> PRGLGPLQIWQTDFTLEPRMA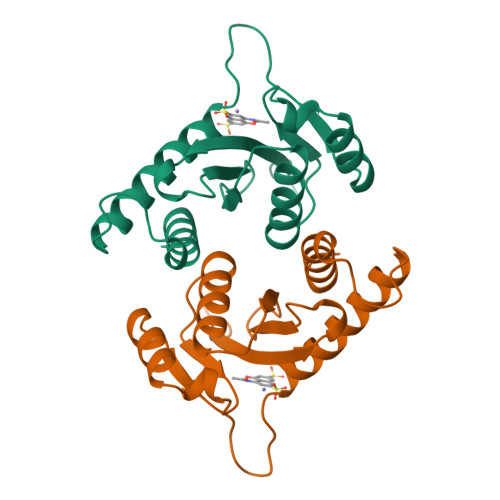PRSWLAVTVDTASSAIVVTQHGRVTSVAAQHHWATAIAVLGRPKAIKTDNGSCFTSKSTREWLARWGIAHTTGIPGNSQGQAMVERANRLLKDKIRVLAEGDGFMKRIPTSKQGELLAKAMYALNHFERGENTKTNL> TKGLVLGIYSKEKEEDEPQFTSAGENFNKLVSGKLREILNISGPPLKAGKTRTFYGLHEDFPSVVVVGLGKKTAGIDEQENWHEGKENIRAAVAAGCRQIQDLEIPSVEVDPCGDAQAAAEGAVLGLYEYDDLKQKRKVVVSAKLHGSEDQEAWQRGVLFASGQNLARRLMETPANEMTPTKFAEIVEENLKSASIKTDVFIRPKSWIEEQEMGSFLSVAKGSEEPPVFLEIHYKGSPNASEPPLVFVGKGITFDSGGISIKAAANMDLMRADMGGAATICSAIVSA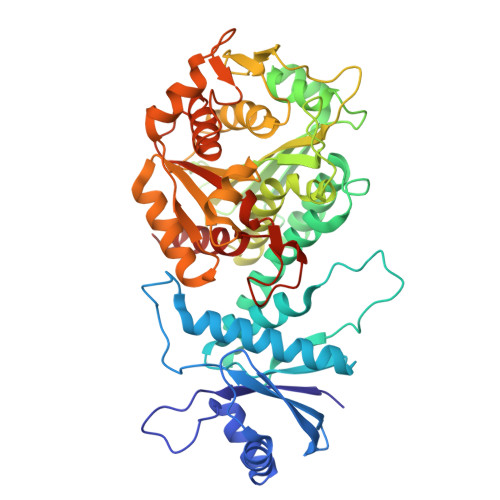AKLDLPINIVGLAPLCENMPSGKANKPGDVVRARNGKTIQVDNTDAEGRLILADALCYAHTFNPKVIINAATLTGAMDIALGSGATGVFTNSSWLWNKLFEASIETGDRVWRMPLFEHYTRQVIDCQLADVNNIGKYRSAGACTAAAFLKEFVTHPKWAHLDIAGVMTNKDEVPYLRKGMAGRPTRTLIEFLFRFSQESA N-[2-[5-(1H-benzimidazol-5-yl)-4H-1,2,4-triazol-3-yl]ethyl]-5-(4-fluorophenyl)-2,3-dihydroxybenzamide | C24 H19 F N6 O3 | 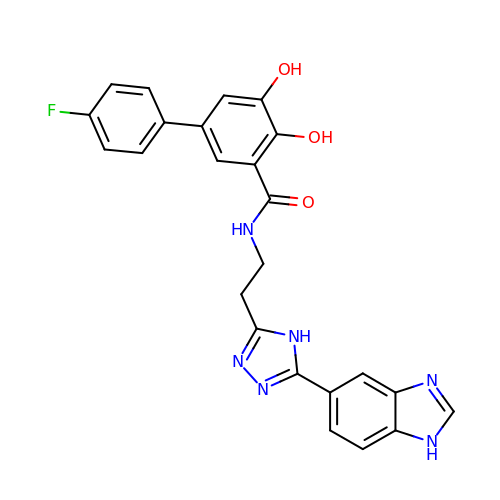JTVOGMMEJFMJHA-UHFFFAOYSA-N>[7x]AIAHIATEYVFSDFLLKDPPESKYKGLRLELAVDKLVSCIAVGLPLLLISLAFAQEITLGSQISCFAPTSFSWRQAAYVDSFCWAAVQQKHLSQSDSGNVPLWLHKFFPYILLLVAVLLYLPNLFWRFTAAPHLSSDLKFVMEELDKCYNRDIKD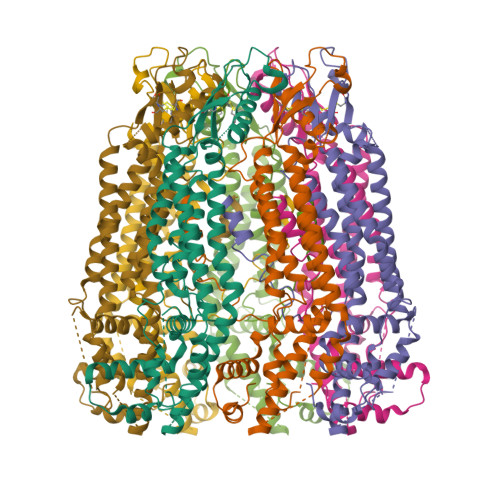IKAANNLNSSDKRDGLNSPVVSENLQQSLWEIPLSHYKYPIVEQYLKTKNNSYGLIIKYLICRVVTLIIVFTACIYLGYYISLFSLTDEFTCNIRTGILRNDTALPPLVQCKLIAVGVFRLLSYINLIIYVLIMPFIIYAMLVPFRKTANVLKVYEVLPTFSVQQAPSKTYDDHSLFLLFLEENVSELKSYKFLKVLENIKNTGENFDTIQYLTSLGTVK>QFQKPGDAIEYRQSAFTLIANHFGRVAAMAQGKAPFDAKVAAENIALVSTLSKLPLTAFGPGTDKGHG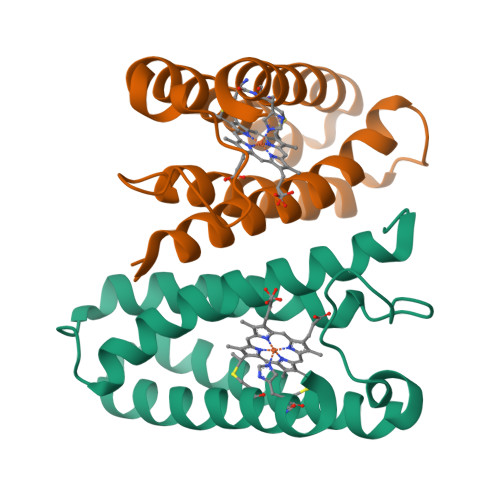TEAKPAVWSDAAGFKAAADKFAAAVDKLDAAGKTGDFAQIKAAVGETGGACKGCHDKFKEK[2x]>MPNIKIFSGSS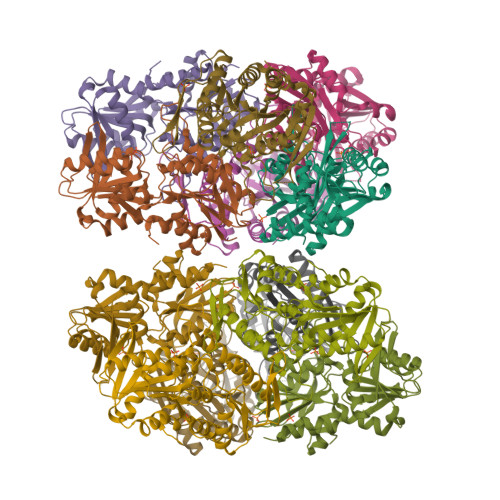HQDLSQKIADRLGLELGKVVTKKFSNQETCVEIGESVRGEDVYIVQSGCGEINDNLMELLIMINACKIASASRVTAVIPCFPYARQDKKDKSRAPISAKLVANMLSVAGADHIITMDLHASQIQGFFDIPVDNLYAEPAVLKWIRENISEWRNCTIVSPDAGGAKRVTSIADRLNVDFALIHKERKKANEVDRMVLVGDVKDRVAILVDDMADTCGTICHAADKLLSAGATRVYAILTHGIFSGPAISRINNACFEAVVVTNTIPQEDKMKHCSKIQVIDISMILAEAIRRTHNGESVSYLFSHVPL[12x]2-[methyl(phenyl)amino]-1-[4-(1H-pyrrolo[2,3-b]pyridin-3-yl)-3,6-dihydropyridin-1(2H)-yl]ethan-1-one 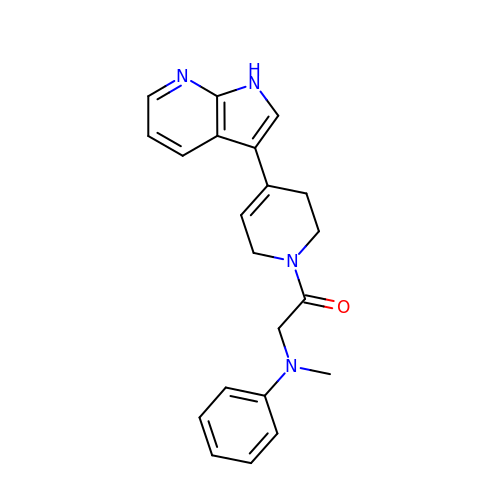| C21 H22 N4 O | YVJWZSCNKWKWOS-UHFFFAOYSA-N> 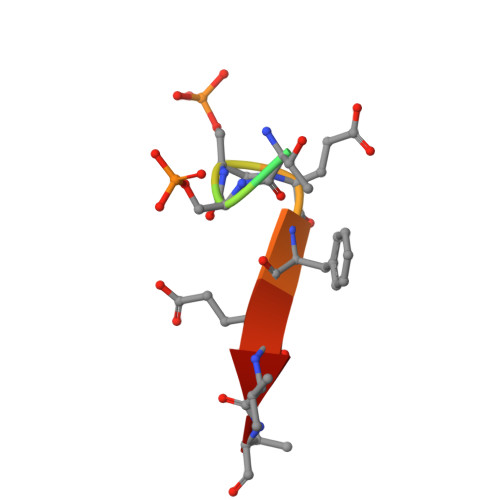SSGTSSEFEVV>[2x]MVDNSRTRPRVGHIQFLSCLPLYWGLARTGTLLDFELTKDTPEKLSEQLVRGDLDIGPVTLVEFLKNADDLVAFPDIAVGCDGPVMSCVIVSQVPLDRLDGARVALGSTSRTSVRLAQLLLSERFGVQPDYYTCPPDLSLMMQEADAAVLIGDAALRANMIDGPRYGLDVHDLGALWKEWTGLPFVFAVWAARRDYAEREPVITRKVHEAFLASRNLSLEEVEK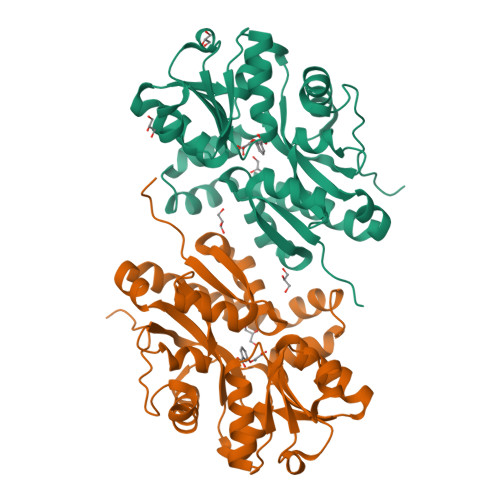VAEQAARWEAFDEDTLAKYFTTLDFRFGAPQLEAVTEFARRVGPTTGFPADVKVELLKPLEHHHHHH>MHIERLAVDESVGRAMPPQRFIEALSDLGVPVEFAGEDEQFGPGDAVASFGHRDAFLDADWVHCIRAGYDEFPVGVYEEAGTYLTNSTGIHGTTVGETVAGYMLTFARRLHAYRDAQHDHAWDLPRYEEPFTLAGERVCVVGLGTLGRGVVDRAAALGMEVVGVRRSGDPVDNVSTVYTPDRLHEAIADARFVVLATPLTDETEGMVAAPEFETMREDASLVNVARGPVVVESDLVAALDSGDIAGAALDVFSEEPLPEDSPLWDFEDVLITPHVSAATSKYHEDVAALIRENIEKIATGDELTNRVV[4x]

Here we describe the molecular basis of the reaction mechanism and dual NADH/NADPH-specificity of D2HDH, a 2-hydroxyacid dehydrogenase from the extreme halophile Haloferax mediterranei, an organism whose proteins have to remain active in high intracellular concentrations of KCl. Sequence analysis has identified D2HDH as a member of the DDH clade of the D-isomer specific 2-hydroxyacid dehydrogenase enzyme family (2HADH), which has potential applications in the synthesis of chiral fine chemicals including alcohols, and hydroxy or amino acids from ketones or ketoacids. Structural studies have shown that all members of this family share a common fold based on two domains, which cycle between open and closed conformational states that serve to close the inter-domain cleft, bringing the substrates together during catalysis. The D2HDH dimer has an overall ellipsoidal appearance in which each monomer is folded into two domains (d1; residues 1–92 and 283–308 and d2; residues 93–282).

Given the presence of a chloride ion in the structure of the D2HDH/NAD+/-2-ketohexanoic acid complex at the 2’ phosphate binding site of NADP+, the decrease in the NADPH-dependent activity of the enzyme at high concentrations of KCl was consistent with the Cl- ion competing with the 2’ phosphate for the same binding site on the protein. Comparing the two structures movements of up to 1.5 Å in the residues of the Arg 165-Val 171 loop, that lies adjacent to the 2’ hydroxyl or 2’ phosphate groups of the two nucleotides, occur. Compared to the loss in activity seen with NADPH at high KCl concentrations, the absence of any similar reduction with NADH is consistent with the independent binding sites for the chloride ion and the 2’ ribose hydroxyl of NADH. At low KCl concentrations the predominant species would be a NADH/enzyme complex, but as the KCl concentration rises, the binding of Cl- at the 2’ phosphate site would increase, to give a NADH/Cl- D2HDH complex which would mimic that of the NADPH enzyme. Three well defined Na+ binding sites per subunit could be confidently assigned, two of which were in common with sites 1 and 3 in the K+ structure. This is possible because the protein ligands in these two sites are clustered together in such a way as to permit the Na+ ion to move closer to them to accommodate its smaller ionic radius, whilst allowing associated differences in the water structure.> GPVCAEASDVYSPCMIASTPPAPFSDVTAVTFDLINGKITPVGDDNWNTHIYNPPIMNVLRTAAWKSGTIHVQLNVRGAGVKRADWDGQVFVYLRQSMNPESYDARTFVI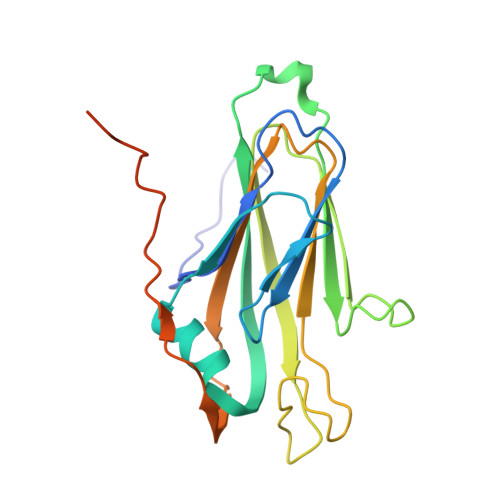SQPGSAMLNFSFDIIGPNSGFEFAESPWANQTTWYLECVATNPRQIQQFEVNMRFDPNFRVAGNILMPPFPLSTETPPLLKFRFRDIERSKRSVMVGHTATAA>MTKIAMYNVSPIEVPYIEDWAKKNDVEIKTTDQALTSATVDLAEGCSSVSLKPLGPVDEEVVYQKLSEYGVKCIGLRIVGFNTINFDWTKKYNLLVTNVPVYSPRAIAEMTVTQAMYLLRKIGEFRYRMDHDHDFTWPSNLISNEIYNLTVGLIGVGHIGSAVAEIFSAMGAKVIAYDVAYNPEFEPFLTYTDFDTVLKEADIVSLHTPLFPSTENMIGEKQLKEMKKSAYLINCARGELVDTGALIKALQDGEIAGAGLDTLAGESSYFGHTGLT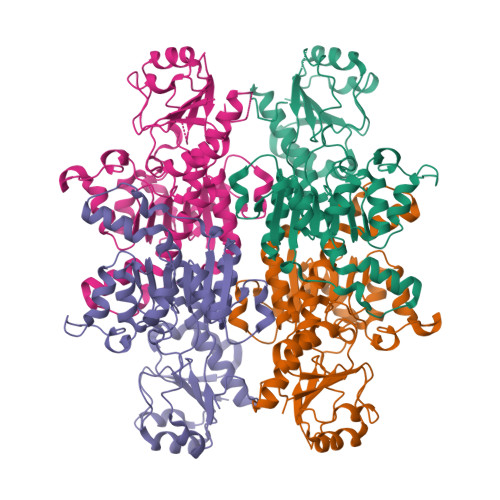DSEIPEDYKTLAKMPNVVITPHSAFYTETSIRNMVQICLTDQLTIAKGGRPRSIVNLTASGHHHHHH[4x]>MSFQGHGIYYIASAYVANTRLALSEDSSANKSPDVIISSDAVDPLNNLWLIEPVGEADTYTVRNAFAGSYMDLAGHAATDGTAIIGYRPTGGDNQKWIISQINDVWKIKSKETGTFVTLLNGDGGGTGTVVGWQNITNNTSQNWTFQKLSQTGANVHATLLACPALRQDFKSYLSDGLYLVLTRDQISSIWQASGLGSTPWRSEIFDCDDFATVFKGAVAKWGNENF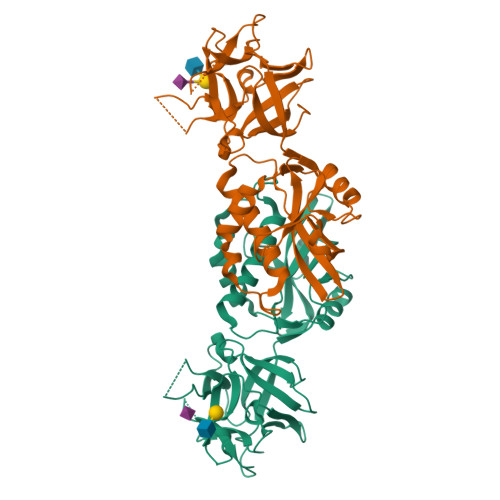KANGFALLCGLMFGSKSSGAHAYNWFVERGNFSTVTFFEPQNGTYSANAWDYKAYFGLF[2x]The first step of the pathway, aldol condensation of phosphoenolpyruvate (PEP) and D-erythrose-4-phosphate (E4P) to 3-deoxy-D-arabino-heptulosonate-7-phosphate (DAHP) is catalyzed by the DAHP synthase enzyme. In B. subtilis, regulation of DAHP synthase is thought to be controlled by its N-terminal domain (BsCM_2), which has residual chorismate mutase activity. Herein, we have reported the crystal structures of the BsCM_2 domain of DAHP synthase from B. subtilis in complex with citrate and chlorogenic acid. A functional trimer has three active sites formed at the interface of two monomers. However, BsCM_2 forms an entirely helical dimeric structure with two active site clefts which are formed by the residue contributions from both monomers, as previously described.

BsCM_2 crystals complexed with citrate (BsCM_2-CIT) and substrate analogue chlorogenic acid (BsCM_2-CGA) diffracted up to 1.9 Å and 1.8 Å resolution, respectively. BsCM_2-CIT and BsCM_2-CGA structures contain four and two monomers per asymmetric unit, respectively. At active site S1, the chlorogenic acid makes hydrogen bonds with the side chain of Arg27, Lys38, Gln86, and the main chain atoms of Arg45, Asp47, and Phe79 of chain B. The ligand molecule also interacts with Lys38, Arg50, and Lys80 of chain B, and Arg10 of chain A through water bridge formation. However, at active site S2, along with the above interactions, the ligand forms a direct hydrogen bond with Lys80 and an additional water bridge-mediated hydrogen bond with Gln86 of chain A. In BsCM_2–CIT structure, the active sites of all the chains were occupied by citrate molecule contributed by crystallization buffer. The citrate molecule interacts with the residues Arg27, Lys38, Asp47 and Gln86 of chain A and Arg10 of adjacent chain B through hydrogen bonding, and similarly in chain C, and chain D. The citrate molecule also makes additional interactions with the residues Arg27, Arg50 and Phe79 via water bridge formation. Position and interactions of the citrate with the protein differ from chlorogenic acid. However, citrate only makes a hydrogen bond with Lys38 and does not have any polar contact with Arg45 and Lys80. Additionally, Phe79 backbone atoms form direct interactions with chlorogenic acid, but form water mediated interaction with citrate. These differences in protein-ligand interactions are likely to be responsible for differences in the binding of ligands with protein as observed in ITC studies. The equilibrium dissociation constant for chorismate, citrate, and chlorogenic acid was calculated as 725 µM, 600 µM and 480 µM, respectively.

>[4x]MSNTELELLRQKADELNLQILKLINERGNVVKEIGKAKEAQGVNRFDPVRERTMLNNIIENNDGPFENSTIQHIFKEIFKAGLELQEEDH>[4x]HHHHHHSSGLVPRGSHMASMSKVGINGFGRIGRLVLRRLLEVKSNIDVVAINDLTSPKILAYLLKHDSNYGPFPWSVDF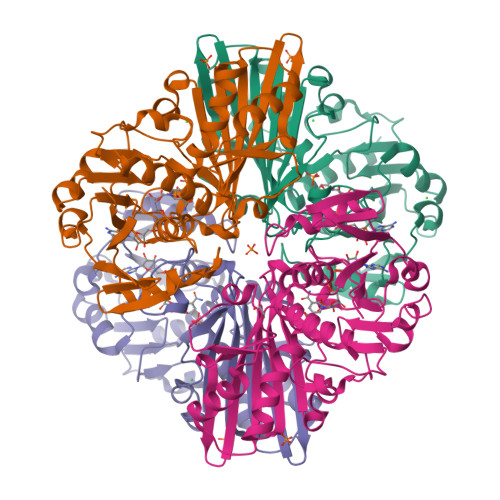TEDSLIVDGKSIAVYAEKEAKNIPWKAKGAEIIVECTGFYTSAEKSQAHLDAGAKKVLISAPAGEMKTIVYNVNDDTLDGNDTIVSVASATTNCLAPMAKALHDSFGIEVGTMTTIHAYTGTQSLVDGPRGKDLRASRAAAENIIPHTTGAAKAIGLVIPELSGKLKGHAQRVPVKTGSVTELVSILGKKVTAEEVNNALKQATTNNESFGYTDEEIVSSDIIGSHFGSVFDATQTEITAVGDLQLVKTVAWYDNEYGFVTQLIRTLEKFAKL> R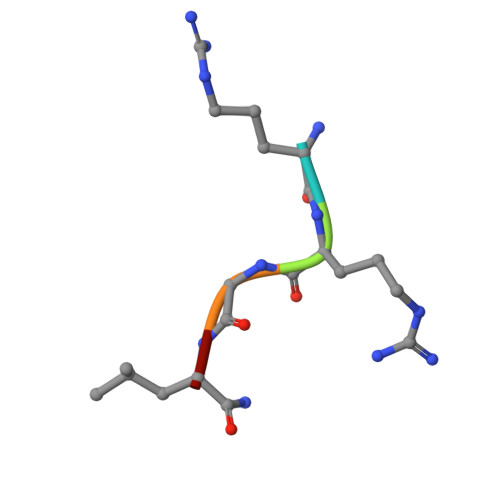RGLX> GPRKAEIMESIKRLYPGSVYGRLIDLCQPTQKKY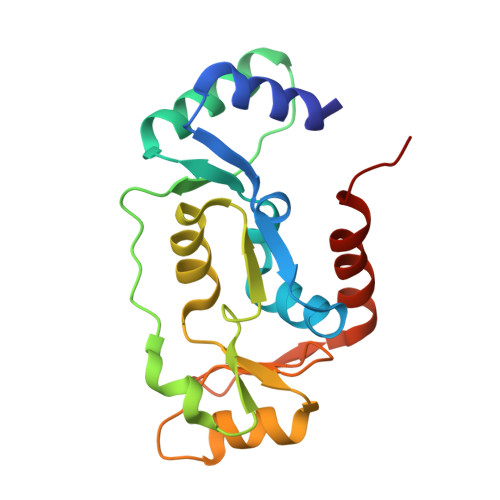QIAVTKVLGKNMDAIIVDSEKTGRDCIQYIKEQRGEPETFLPLDYLEVKPTDEKLRELKGAKLVIDVIRYEPPHIKKALQYACGNALVCDNVEDARRIAFGGHQRHKTVALDGTLFQKSGVISGGASDLKAKARRWDEKAVDKLK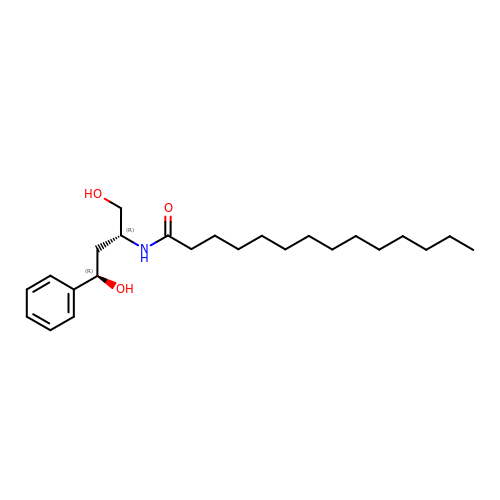N-[(1R,3R)-3-hydroxy-1-(hydroxymethyl)-3-phenylpropyl]tetradecanamide | C24 H41 N O3 | MWVNSXPNTJYJDR-DHIUTWEWSA-N QCs belong to the family of aminoacyltransferases and catalyze the cyclization of N-terminal glutamine/glutamate residues of peptides and proteins with concomitant release of ammonia/water. Glutaminyl cyclases (QCs) from the oral pathogens Porphyromonas gingivalis, Tannerella forsythia, and Prevotella intermedia represent attractive target enzymes for small-molecule inhibitor development, as their action is likely to stabilize essential periplasmic and outer membrane proteins by N-terminal pyroglutamination. Crystal structures of the enzymes from P. gingivalis (PgQC) and T. forsythia (TfQC) reveal a tertiary structure composed of an eight-stranded β-sheet surrounded by seven α-helices, typical of animal type II QCs. In each case, an active site Zn ion is tetrahedrally coordinated by conserved residues.

The same architecture is observed for TfQC, with an r.m.sd to PgQC of 1.1 Å for 286 Cα atoms. The only significant differences are seen in an altered course of the loop between α4 and βD (“4-D loop”, presumably due to the presence of TfPro171) and a lengthened loop connecting βD and α6 (“Tf insertion loop”, which starts with conserved residues PgAsp183 and ends with PgTrp193). A small degree of structural variation is observed between two sets of crystallographically independent TfQC monomers in the loop containing TfGly268-Gly269 that connects βG and α8, which was also observed for mouse QC (MmQC). Interestingly, two distinct conformations of the loop connecting α6 and βE (“6-E loop”) were observed in TfQC: the TfVal212–Pro213 peptide bond adopts a cis-conformation in two of the monomers as opposed to the trans-conformation found in PgQC, leading to an alternative orientation of α6.

>GSHMGQKNTTKEETTEPADTDKRIEAPTFNADSAYAYIERQVAFGPRVPNTEAHQRCADYLAGELDRHGAKVYVQEAVLTAYNGEKLKAQNIVGAFQPEKSRRVLLFAHWDSRPYADHDTDEANHRKPIDGADDGGSGVGILLEIARQIQAKAPAIGIDIVFFDAEDYGTPEFVDEYKPDTWCLGSQFWAKNPHVPNYKAEFGILLDMVGSRGATFYKESTSVQYAARYVEKVWTAARELGYGKYFINAQGGAIVDDHQYVIQGLRTPCLDIINYDPDTQSGFGPYWHTQNDTMENIDRETLKAVGETILNVIYNEK[4x]> MGIDINTKIFNSVAEVFQKAQGSYAGHRKHIAVLKKIQSKAVEQGYEDAFNFWFDKLVTKILPLKKNEIIDRIVKLVAAFIASLERELILAKKQNYKLTNDEEGIFSRFVDQFIRHVLRGVESPDKNVRFRVLQLLAVIMDNIGEIDESLFNLLILSLNKRIYDREPTVRIQAVFCLTKFQDEEQTEHLTELSDNEENFEATRTLVASIQNDPSAEVRRAAMLNLINDNNTRPYILERARDVNIVNRRLVYSRILKSMGRKCFDDIEPHIFDQLIEWGLEDRELSVRNACKRLIAHDWLNALDGDLIELLEKLDVSRSSVCVKAIEALFQSRPDILSKIKFPSIWKDFTVEIAFLFRAIYLYCLDNNITEMLEENFPEASKLSEHLNHYILLRYHHNDISNDSQSHFDYNTLEFIIEQLSIAAERYDYSDEVGRRSMLTVVRNMLALTTLSEPLIKIGIRVMKSLSINEKDFVTMAIEIINDIRDDDIEKQESESDIINNLPPEKEASSATIVLCLTRSSYMLELVNTPLTENILIASLMDTLITPAVRNTAPNIRELGVKNLGLCCLLDVKLAIDNMYILGMCVSKGNASLKYIALQVIVDIFSVHGNTVVDGEGKVDSISLHKIFYKVLKNNGLPECQVIAAEGLCKLFLADVFTDDDLFETLVLSYFSPINSSNEALVQAFAFCIPVYCFSHPAHQQRMSRTAADILLRLCVLWDDLQSSVIPEVDREAMLKPNIIFQQLLFWTDPRNLVNQTGSTKKDTVQLTFLIDVLKIYAQIEKKEIKKMIITNINAIFLSSEQDYSTLKELLEYSDDIAENDNLDNVSKNALDKLRNNLNSLIEEINERSETQTKDENNTANDQYSSILGN;> GPLGHMSIFEKDLMAYFDENLNRNWRGREHWKVRNFKKANLVNKESDLLEETRTTIGDTTDKNTTDDKSMDTKKKHKQKKVLEIDFFKTDDSFEDKVFASKGRTKIDMPIKNRKNDTHYLLPDDFHFSTDRITRLFIKPGQKMSLFSHRKHT

Condensin protein complexes coordinate the formation of mitotic chromosomes and thereby ensure the successful segregation of replicated genomes. Here, we identify a direct DNA-binding site in the eukaryotic condensin complex, which is formed by its Ycg1Cnd3 HEAT-repeat and Brn1Cnd2 kleisin subunits. A peptide loop of the kleisin subunit encircles the bound DNA and, like a safety belt, prevents its dissociation. Firm closure of the kleisin loop around DNA is essential for the association of condensin complexes with chromosomes and their DNA-stimulated ATPase activity.

To unambiguously determine the position and orientation of DNA bound to the Ycg1–Brn1 subcomplex, we solved the co-crystal structure of Sc Ycg1–Brn1 with 18-bp dsDNA to 2.98 Å resolution. As expected from the surface charge distribution and the results of the mutation experiments, we detected additional electron density corresponding to a DNA double helix within the Ycg1–Brn1 groove. In the crystal, DNA duplexes pack via base-stacking interactions, with one copy of Ycg1–Brn1 contacting two-thirds of one DNA molecule and one-third of a symmetry-related DNA molecule. The DNA helix is unwound by ∼65 degrees over 11 bp and bent by 7 degrees at one end, which results in an offset in the end-to-end stacking arrangement. This conformation is most likely necessary to compensate for the fact that the 18-bp DNA is slightly too long for the 1.5 helical turns required to produce the 21-screw axis observed in the crystal and is not a consequence of binding to Ycg1–Brn1. Several conserved basic residues of both protein subunits, including those we had mutated (Sc Ycg1K70, K71, Sc Ycg1K849, Sc Brn1K409, R411, and Sc Brn1K456 corresponding to Ct Ycg1K100, K101, Ct Ycg1K917, Ct Brn1R539, R541, and Ct Brn1K559), interact with the phosphate backbone of both DNA strands. Comparison of free and DNA-bound structures shows that Ycg1 and Brn1 undergo fairly minor conformational changes upon DNA binding. In addition to a slight shift of the N- and C-terminal shoulders of Ycg1, the most notable difference upon DNA binding is the reorientation toward the double helix of residues within the α1 latch segment of Brn1, including two positively charged residues of the BC1 patch (Sc Brn1K409 and Sc Brn1R411). The change in the conformation of the latch segment might either help to stabilize DNA binding or alter the affinity between the latch and the buckle. The latter hypothesis is consistent with the formation of hydrophobic contacts between a valine residue located between the two charged residues (Sc Brn1V410) and the buckle residues (Sc Ycg1F808 and Sc Brn1W408) in the DNA-bound structure.> MAWATTFYNVFVKRNSAFVATILASAFVFDMTFETAI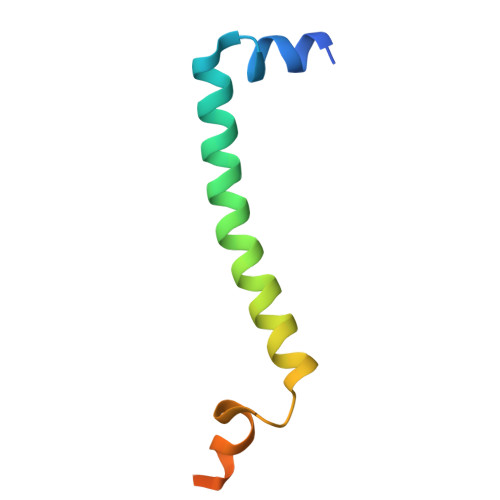DNFWDRINAGKQWKDIRHKYIEAAGDDDEDDE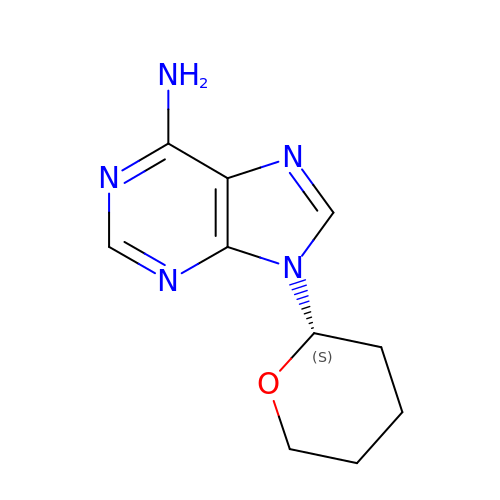9-[(2~{S})-oxan-2-yl]purin-6-amine | C10 H13 N5 O | ATNWAGKQIUHFQP-ZETCQYMHSA-N>SMQEKDASSQGFLPHFQHFATQAIHVGQDPEQWTSRAVVPPISLSTTFKQGAPGQHSGFEYSRSGNPTRNCLEKAVAALDGAKYCLAFASGLAATVTITHLLKAGDQIICMDDVYGGTNRYFRQVASEFGLKISFVDCSKIKLLEAAITPETKLVWIETPTNPTQKVIDIEGCAHIVHKHGDIILVVDNTFMSPYFQRPLALGADISMYSATKYMNGHSDVVMGLVSVNCESLHNRLRFLQNSLGAVPSPIDCYLCNRGLKTLHVRMEKHFKNGMAVAQFLESNPWVEKVIYPGLPSHPQHELVKRQCTGCTGMVTFYIKGTLQHAEIFLKNLKLFTLAESLGGFESLAELPAIMTHASVLKNDRDVLGISDTLIRLSVGLEDEEDLLEDLDQAL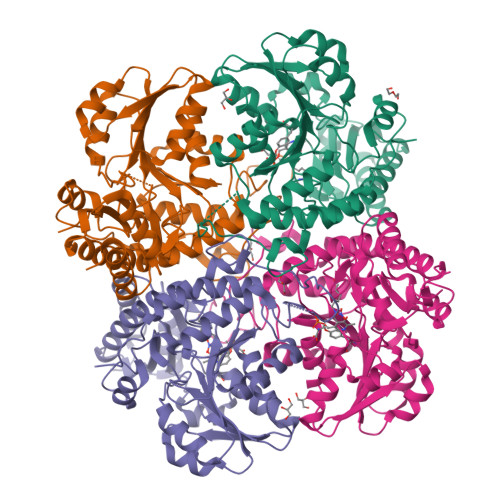KAAHPPSG[4x]> MEVNVKGNYVQVYVMLPLDAVSVNNRFEKGDELRAQLRKLVEAGVDGVMVDVWWGLVEGKGPKAYDWSAYKQLFELVQKAGLKLQAIMSFHQCGGNVGDAVNIPIPQWVRDVGTRDPDIFYTDGHGTRNIEYLTLGVDNQPLFHGRSAVQMYADYMTSFRENMKEFLDAGVIVDIEVGLGPAGEMRYPSYPQSHGWSFPGIGEFICYDKYLQADFKAAAAAVGHPEWEFPNDVGQYNDTPERTQFFRDNGTYLSEKGRFFLAWYSNNLIKHGDRILDEA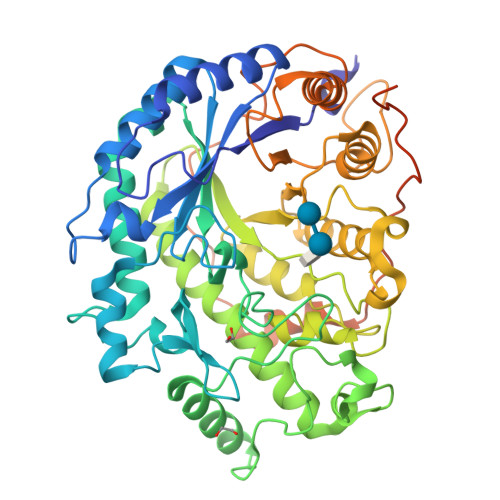NKVFLGYKVQLAIKISGIHWWYKVPSHAAELTAGYYNLHDRDGYRTIARMLKRHRASINFTCAEMRDSEQSSQAMSAPEELVQQVLSAGWREGLNVACENALPRYDPTAYNTILRNARPHGINQSGPPEHKLFGFTYLRLSNQLVEGQNYANFKTFVDRMHANLPRDPYVDPMAPLPRSGPEISIEMILQAAQPKLQPFPFQEHTDLPVGPTGGMGGQAEGPTCGMGGQVKGPTGGMGGQAEDPTSGIGGELPATM> MGKALVIVESPAKAKTINKYLGSDYVVKSSVGHIRDLPTSGSAAKKSADSTSTKTAKKPKKDERGALVNRMGVDPWHNWEAHYEVLPGKEKVVSELKQLAEKADHIYLATDLDREGEAIAWHLREVIGGDDARYSRVVFNEITKNAIRQAFNKPGELNIDRVNAQQARRFMDRVVGYMVSPLLWKKIARGLSAGRVQSVAVRLVVEREREIKAFVPEEFWEVDASTTTPSGEALALQVTHQNDKPFRPVNKEQTQAAVSLLEKARYSVLEREDKPTTSKPGAPFITSTLQQAASTRLGFGVKKTMMMAQRLYEAGYITYMRTDSTNLSQDAVNMVRGYISDNFGKKYLPESPNQYASKENSQEAREAIRPSDVNVMAESLKDMEADAQKLYQLIWRQFVACQMTPAKYDSTTLTVGAGDFRLKARGRILRFD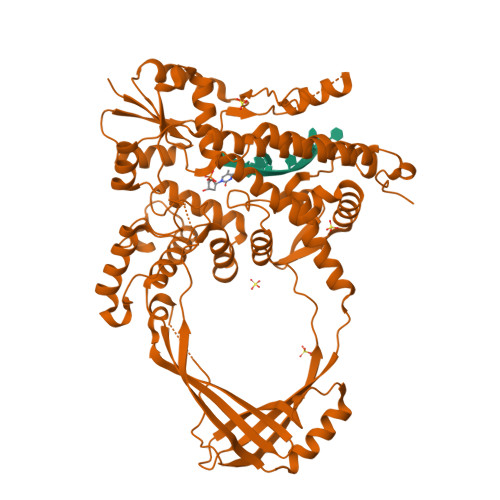GWTKVMPALRKGDEDRILPAVNKGDALTLVELTPAQHFTKPPARFSEASLVKELEKRGIGRPSTYASIISTIQDRGYVRVENRRFYAEKMGEIVTDRLEENFRELMNYDFTAQMENNLDQVANHEAEWKAVLDHFFSDFTQQLDKAEKDPEEGGMRPNQM>[2x]HHNKVRTCWNEGRPALAGWLQLPGTLHAEALARLDYDAVVIDMQHSPIDFGQVAPMLIAIELGGAEPFVRTQVNDPSDIMKLLDAGAYGIIAPMVNTRAEAQTLASALHYSPRGLRSFGPRRPSLRYGSGYLAQASETVVGLAMIETREALANIDEILSVDGIDGVFIGPTDLALDLGHAPLVDTEEAEVVSAIAHVRERAHAA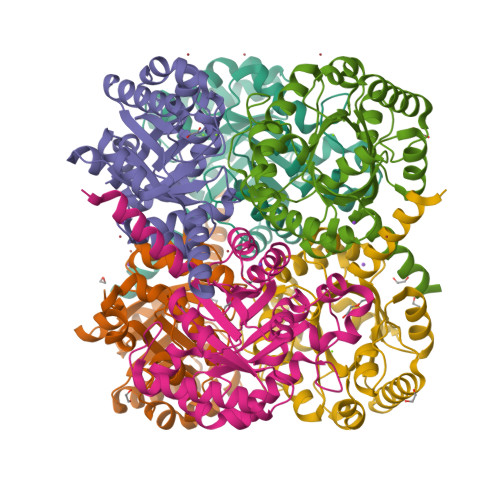GKRVGIWCGSGGFARVKLAEGFDFVTAAPDLAMLSAAARQVIADARAL> ASKGTSHEAGIVCRITKPALLVLNHETAKVIQTAFQRASYPDITGEKAMMLLGQVKYGLHNIQISHLSIASSQVELVEAKSIDVSIQDVSVVFKGTLKYGYTTAWWLGIDQSIDFEIDSAIDLQINTQLTADSGRVRTDAPDCYLSFHKLLLHLQGEREPGWIKQLFTNFISFTLKLVLKGQICKEINVISNIMADFVQTRAASILSDGDIGVDISLTGDPVITASYLESHHKGHFIYKDVSEDLPLPTFSPTLLGDSRMLYFWFSERVFHSLAKVAFQDGRLMLSLMGDEFKAVLETWGFNTNQEIFQEVVGGFPSQAQVTVHCLKMPKISCQNKGVVVDSSVMVKFLFPRPDQQHSVAYTFEEDIVTTVQASYSKKKLFLSLLDFQITPKTVSNLTESSSESIQSFLQSMITAVGIPEV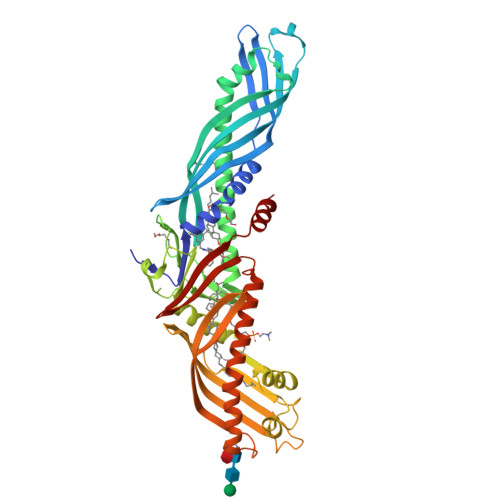MSRLEVVFTALMNSKGVSLFDIINPEIITRDGFLLLQMDFGFPEHLLVDFLQSLS>[12x]MLEDGFSYKTIGEIQRRRGNLWFRTYQRYLFSLAYQMFEWQGLPKTVDPIFLEKQLHQRGFVAFYKDEMYGYLGVQGTLSGQINLYNQPNFYTASAPTYQKSFPLYWYDMGEDLNEKGQGIVIYNNLERMPTLDILNLYAMNLAELKETIYVNQNAQKTPVIIKAGDNDLFSMKQVYNKYEGNEPVIFAGKKFNTDDIEVLKTDAPYVADKLTMLFKDQWNEAMTFLGLSNANTDKKERLIQSEVESNNDQIQGSANIYLAPRQEACRLINEYYGLNVSVKLRKELVGNGELHNAIEGNSGMGNTV

The Portal Protein (PP) complex is a central component of Caudovirales virions in the process of self-assembly of phages. The PP has multiple functions: (1) as a nucleation point for capsid formation; (2) as part of the motor for loading the genome into the capsid; (3) as a head-full sensor; and (4) as a conduit for genome translocation. All portal protein primary structures are characterised by a common fold comprising four conserved domains: The capsid-facing C-terminal crown, the interior wing and stem, and the tail-facing clip domains. Using cryoEM, we determined the structures of two portal proteins: GA1 gp10, and phiCPV4 gp17, which are phages of the Salasmaviridae and Guelinviridae families respectively. Both GA1 gp10 and phiCPV4 gp17 PPs have the canonical fold and domain organisation found in the portal protein phi29 gp10.

The GA1 phage of the Salasmaviridae family targets the pathogen Bacillus pumilus, causative of serious infant infections. The GA1 PP (gp10) has 52.4% sequence identity with the phi29 PP (gp10). For GA1 gp10 the tag had to be proteolytically cleaved to prevent the formation of rosettes and the buffer pH adjusted, to obtain sufficient oligomeric particles for cryo-EM (Materials and Methods Section 2.2). The GA1 gp10 dodecamer has a height of 78 Å and the outer diameter of 152 Å. Assessment of structural similarity of the wing domains between GA1 gp10 and phi29 gp10 RSMD in aligned atomic models demonstrated that wings in GA1 and phi29 PP have nearly identical folds, which is not surprising considering that they have a very high percentage (52.4%) of sequence identity. The N-terminus of GA1 gp10 is relatively well defined in the EM map and could be traced from residue Tyr8. The N-terminus forms two helical elements on the outer part of the PP complex where the short α0-helix comprises residues Tyr8 to Arg18 and is positioned in a horizontal orientation with respect to the central axis of the PP. Arg18 forms a salt bridge with Glu148 of the adjacent subunit. In GA1 gp10, four hydrogen bonds are located between the α3 helices of the neighbouring subunits Tyr139A, Thr149A, Gln154B, Lys147B. However, there are interesting differences in the arrangement of the clip domain between the phages: GA1 gp10 has a beta sheet formed by β8 and β10 strands from one subunit and the third β9 located on the outer edge of the beta sheet is from the adjacent subunit.Utp22 and Rrp7, two interacting proteins with no recognizable domain, are components of the 90S preribosome or the small subunit processome that conducts early processing of 18S rRNA. Utp22 and Rrp7 are two proteins associated with early 90S preribosomes and form the UTP-C complex together with four subunits of casein kinase 2. Like most early-acting SSU synthesis factors, Utp22 and Rrp7 are required for early processing of 18S rRNA and 40S ribosome formation. Here, we determine the cocrystal structure of Utp22 and Rrp7 complex at 1.97 Å resolution and the NMR structure of a C-terminal fragment of Rrp7, which is not visible in the crystal structure.

The full-length proteins of yeast Utp22 and Rrp7 were coexpressed using recombinant baculoviruses in insect cells and then copurified and cocrystallized. N-terminal residues 1–80 of Utp22, C-terminal residues 190–297 of Rrp7, and several internal loops of each protein were not visible in the crystal structure, likely due to structural flexibility. Utp22 and Rrp7 form a 1∶1 dimer that adopts a saddle-like structure with approximate dimensions of 137 Å×66 Å×69 Å. The N-terminal half (N-half) and C-terminal half (C-half) of Utp22 are structurally similar to each other and are arranged in tandem along the longest dimension. Rrp7 binds at the C-half of Utp22, forming a raised end. The structure of Utp22 can be divided into eight domains (D1 though D8). Both the N-half (D1–D4, residues 81–689) and C-half (D5–D8, residues 699–1237) are structurally similar to class I CCA-adding enzyme in all four individual domains. Utp22 is likewise an intramolecular dimer composed of two copies of CCA-adding enzyme modules. In addition, several structural elements in D1 and D5, including the loop between β5 and α6, the N-terminal part of α6, α20, and the N-terminal part of α21 would occlude the RNA-binding paths in both halves of Utp22 and prevent access of substrate tRNA to the active site. These structural observations indicate that Utp22 is inactive as a CCA-adding enzyme. The NTD adopts a two-layered α/β fold, which is similar to the fold of RRM according to DALI search (best z-score = 4.8). The NTD and linker region of Rrp7 associate with D6, D7, and D8 of Utp22 through an extensive interface, which buries 3,116 Å2 of solvent accessible surface area per subunit.

> MATSVKRKASETSDQNIVKVQKKHSTQDSTTDNGSKENDHSSQAINERTVPEQENDESDTSPESNEVATNTAATRHNGKVTATESYDIHIARETAELFKSNIFKLQIDELLEQVKLKQKHVLKVEKFLHKLYDILQEIPDWEEKSLAEVDSFFKNKIVSVPFVDPKPIPQNTNYKFNYKKPDISLIGSFALKAGIYQPNGSSIDTLLTMPKELFEKKDFLNFRCLHKRSVYLAYLTHHLLILLKKDKLDSFLQLEYSYFDNDPLLPILRISCSKPTGDSLSDYNFYKTRFSINLLIGFPYKVFEPKKLLPNRNCIRIAQESKEQSLPATPLYNFSVLSSSTHENYLKYLYKTKKQTESFVEATVLGRLWLQQRGFSSNMSHSGSLGGFGTFEFTILMAALLNGGGINSNKILLHGFSSYQLFKGVIKYLATMDLCHDGHLQFHSNPENSSSSPASKYIDEGFQTPTLFDKSTKVNILTKMTVSSYQILKEYAGETLRMLNNVVQDQFSNIFLTNISRFDNLKYDLCYDVQLPLGKYNNLETSLAATFGSMERVKFITLENFLAHKITNVARYALGDRIKYIQIEMVGQKSDFPITKRKVYSNTGGNHFNFDFVRVKLIVNPSECDKLVTKGPAHSETMSTEAAVFKNFWGIKSSLRRFKDGSITHCCVWSTSSSEPIISSIVNFALQKHVSKKAQISNETIKKFHNFLPLPNLPSSAKTSVLNLSSFFNLKKSFDDLYKIIFQMKLPLSVKSILPVGSAFRYTSLCQPVPFAYSDPDFFQDVILEFETSPKWPDEITSLEKAKTAFLLKIQEELSANSSTYRSFFSRDESIPYNLEIVTLNILTPEGYGFKFRVLTERDEILYLRAIANARNELKPELEATFLKFTAKYLASVRHTRTLENISHSYQFYSPVVRLFKRWLDTHLLLGHITDELAELIAIKPFVDPAPYFIPGSLENGFLKVLKFISQWNWKDDPLILDLVKPEDDIRDTFETSIGAGSELDSKTMKKLSERLTLAQYKGIQMNFTNLRNSDPNGTHLQFFVASKNDPSGILYSSGIPLPIATRLTALAKVAVNLLQTHGLNQQTINLLFTPGLKDYDFVVDLRTPIGLKSSCGILSATEFKNITNDQAPSNFPENLNDLSEKMDPTYQLVKYLNLKYKNSLILSSRKYIGVNGGEKGDKNVITGLIKPLFKGAHKFRVNLDCNVKPVDDENVILNKEAIFHEIAAFGNDMVINFETD;> MGIEDISAMKNGFIVVPFKLPDHKALPKSQEASLHFMFAKRHQSSNSNESDCLFLVNLPLLSNIEHMKKFVGQLCGKYDTVSHVEELLYNDEFGLHEVDLSALTSDLMSSTDVNEKRYTPRNTALLKFVDAASINNCWNALKKYSNLHAKHPNELFEWTYTTPSFTTFVNFYKPLDIDYLKEDIHTHMAIFEQREAQAQEDVQSSIVDEDGFTLVVGKNTKSLNSIRKKILNKNPLSKHENKAKPISNIDKKAKKDFYRFQVRERKKQEINQLLSKFKEDQERIKVMKAKRKFNPYT>GGGTPKAPNLEPPLPEEEKEGSDLRPVVIDGSNVAMSHGNKEVFSCRGILLAVNWFLERGHTDITVFVPSWRKEQPRPDVPITDQHILRELEKKKILVFTPSRRVGGKRVVCYDDRFIVKLAYESDGIVVSNDTYRDLQGERQEWKRFIEERLLM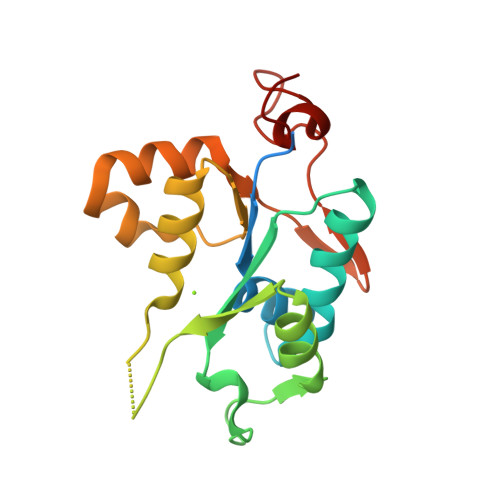YSFVNDKFMPPDDPLGRHGPSLDNFLRKKP[2x]> MKIIILGAGQVGGTLAENLVGENNDITIVDNNADRLRELQDKYDLRVVNGHASHPDVLHEAGAQDADMLVAVTNTDETNMAACQVAFTLF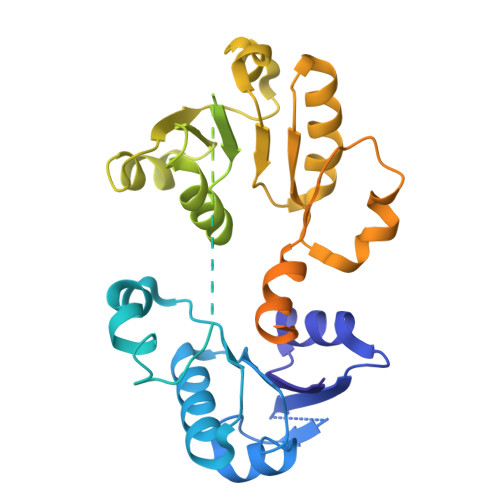NTPNRVARIRSPEYLAEKEALFKSGAIPVDHLIAPEELVTSYIERLIQYPGALQVVSFAEQKVSLVAVKAYYGGPLVGNALSALREHMPHIDTRVAAIFRQGRPIRPQGTTIIEADDEVFFVAASNHIRSVMSELQRLEKPYRRIMIVGGGNIGASLAKRLEQTYSVKLIERDYQRAEKLSEQLENTIVFCGDAADQELLTEENIDQVDVFIALTNEDETNIMSAMLAKRMGAKKVMVLIQRGAYVDLVQGGVIDVAISPQQATISALLTHVRRADIVNVSSLRRGAAEAIEAVAHGDETTSKVVGRAIGDIKLPPGTTIGAVVRGEEVLIAHDRTVIEQDDHVVMFLVDKKYVPDVEALFQPSPFFL>[2x]LADSIVPRQQWAAIEPRRQIKMNGRADEIFLWQTGPDTCSLMGLTADKCQGCLQDSSCTEQIVKALQDADFKEGNDDIKYNFLIDQDGVIYEGR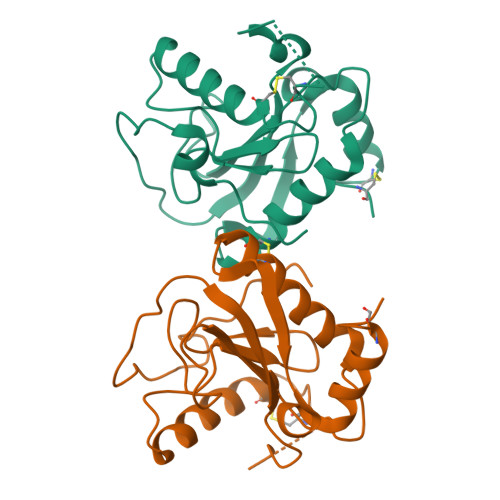GWGVVGQHTKGRDSHSIGVAVIGDFGKKEPSQALQDALSKLIICGQAAEELSSGARLRTTPAMSGQAFYDMLDRCDGLCLDD>GPGSMDWYVGTEWEDKNRGLAKKVIGLQFTEMDKPTIISTVEFSVNKKATNLGGRPSKYLVSDESATYPQKHSLEMGTSLTAVDCYLELLLQQFVPGETAACSITTKTGERIEF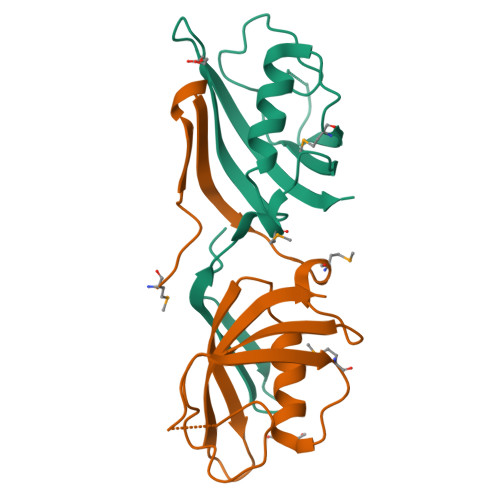ELKLEKIVKN[2x]> VTSVEQRTATAVFSRTGSRMAERRLAFMLVAPAAMLMVAVTAYPIGYALWLSLQRNNLATPNDTAFIGLGNYHTILIDRYWWTALAVTLAITAVSVTIEFVLGLALALVMHRTLIGKGLVRTAVLIPYGIVTVVASYSWYYAWTPGTGYLANLLPYDSAPLTQQIPSLGIVVIAEVWKTTPFMSLLLLAGLALVPEDLLRAAQVDGASAWRRLTKVILPMIKPAIVVALLFRTLDAFRIFDNIYVLTGGSNNTGSVSILGYDNLFKGFNVGLGSAISVLIFGCVAVIAFIFIKLFGAAAPGGEPSGR;> VGARRATYWAVLDTLVVGYALLPVLWIFSLSLKPTSTVKDGKLIPSTVTFDNYRGIFRGDLFSSALINSIGIGLITTVIAVVLGAMAAYAVARLEFPGKRLLIGAALLITMFPSISLVTPLFNIERAIGLFDTWPGLILPYITFALPLAIYTLSAFFREIPWDLEKAAKMDGATPGQAFRKVIVPLAAPGLVTAAILVFIFAWNDLLLALSLTATKAAITAPVAIANFTGSSQFEEPTGSIAAGAIVITIPIIVFVLIFQRRIVAGLTSGAVKG;>[2x]MAEIVLDHVNKSYPDGHTAVRDLNLTIADGEFLILVGPSGCGKTTTLNMIAGLEDISSGELRIAGERVNEKAPKDRDIAMVFQSYALYPHMTVRQNIAFPLTLAKMRKADIAQKVSETAKILDLTNLLDRKPSQLSGGQRQRVAMGRAIVRHPKAFLMDEPLSNLDAKLRVQMRGEIAQLQRRLGTTTVYVTHDQTEAMTLGDRVVVMYGGIAQQIGTPEELYERPANLFVAGFIGSPAMNFFPARLTAIGLTLPFGEVTLAPEVQGVIAAHPKPENVIVGVRPEHIQDAALIDAYQRIRALTFQVKVNLVESLGADKYLYFTTESPAVHSVQLDELAEVEGESALHENQFVARVPAESKVAIGQSVELAFDTARLAVFDADSGA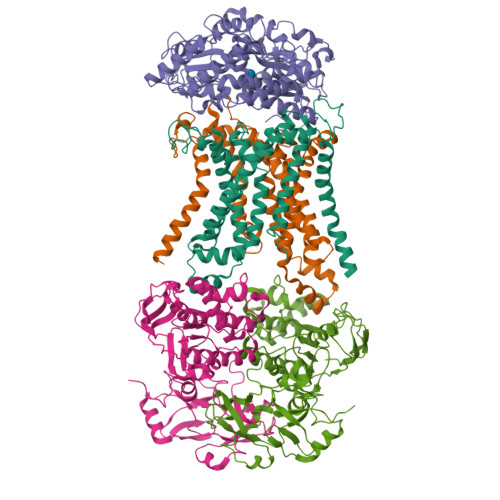NLTIPHRA;> VVMSRGRIPRLGAAVLVALTTAAAACGADSQGLVVSFYTPATDGATFTAIAQRCNQQFGGRFTIAQVSLPRSPNEQRLQLARRLTGNDRTLDVMALDVVWTAEFAEAGWALPLSDDPAGLAENDAVADTLPGPLATAGWNHKLYAAPVTTNTQLLWYRPDLVNSPPTDWNAMIAEAARLHAAGEPSWIAVQANQGEGLVVWFNTLLVSAGGSVLSEDGRHVTLTDTPAHRAATVSALQILKSVATTPGADPSITRTEEGSARLAFEQGKAALEVNWPFVFASMLENAVKGGVPFLPLNRIPQLAGSINDIGTFTPSDEQFRIAYDASQQVFGFAPYPAVAPGQPAKVTIGGLNLAVAKTTRHRAEAFEAVRCLRDQHNQRYVSLEGGLPAVRASLYSDPQFQAKYPMHAIIRQQLTDAAVRPATPVYQALSIRLAAVLSPITEIDPESTADELAAQAQKAIDGMGLLP>[2x]GPGSRYPVRRLPFSTVSKQDLAAFERIVPGGVVTDPEALQAPNVDWLRTLRGCSKVLLRPRTSEEVSHILRHCHERNLAVNPQGGNTGMVGGSVPVFDEIILSTARMNRVLSFHSVSGILVCQAGCVLEELSRYVEERDFIMPLDLGAKGSCHIGGNVATNAGGLRFLRYGSLHGTVLGLEVVLADGTVLDCLTSLRKDNTGYDLKQLFIGSEGTLGIITTVSILCPPKPRAVNVAFLGCPGFAEVLQTFSTCKGMLGEILSAFEFMDAVCMQLVGRHLHLASPVQESPFYVLIETSGSNAGHDAEKLGHFLEHALGSGLVTDGTMATDQRKVKMLWALRERITEALSRDGYVYKYDLSLPVERLYDIVTDLRARLGPHAKHVVGYGHLGDGNLHLNVTAEAFSPSLLAALEPHVYEWTAGQQGSVSAEHGVGFRKRDVLGYSKPPGALQLMQQLKALLDPKGILNPYKTLPSQAHHHHHH

Human D-2-HGDH is a member of the 2-hydroxy acid dehydrogenase subfamily of the VAO/PCMH flavoprotein family. Regardless of their promiscuous metabolic origins, D-2-HG and L-2-HG can be converted back to 2-OG by two mitochondrial enzymes in humans, namely D-2-HG and L-2-HG dehydrogenases (D-2-HGDH and L-2-HGDH). Like other members of the VAO/PCMH flavoprotein family, D-2-HGDH is comprised of two major domains named the FAD-binding domain and the substrate-binding domain supplemented with a small C-terminal domain. The active site resides at the interface of the FAD-binding domain and the substrate-binding domain, and consists of the FAD-binding site and the substrate-binding site.

In the apo structure, the substrate-binding site is occupied by several water molecules; in the D-2-HG-bound structure, there are a Zn2+ and a D-2-HG bound at the substrate-binding site. The structural comparison shows that the binding of Zn2+ and D-2-HG at the active site does not induce notable conformational changes in the overall structure and at the FAD-binding site, and hence does not affect the conformation of FAD and its interactions with the protein. The structural comparison shows that the binding of Zn2+ and D-2-HG does not induce notable conformational changes at the substrate-binding site as well except for Glu475 which adopts a different side-chain conformation to interact with the Zn2+. The Zn2+ is coordinated by six ligands, including the side chains of His434, His441, and Glu475, the O4 atom of FAD, and the C1-carboxyl and C2-hydroxyl of D-2-HG. The lactate moiety of D-2-HG is positioned in parallel to the isoalloxazine ring of FAD and the acetate moiety is extended into the deep end of the substrate-binding pocket; both moieties are recognized by several conserved residues. Specifically, the C1-carboxyl of D-2-HG forms several hydrophilic interactions with the side chains of Arg386, Thr390, His434, and His441, two hydrogen bonds with the O4 atom of FAD and a water molecule (Wat1), and a coordination bond with the Zn2+. The C2-hydroxyl of D-2-HG forms hydrogen bonds with the side chains of His441, Glu475, and His476, and a coordination bond with the Zn2+. The C5-carboxyl of D-2-HG forms a salt bridge with the side chain of Lys401 and four hydrogen bonds with the side chains of Thr390, Tyr432, and Asn443, and a water molecule (Wat2). In particular, the O4 atom of the isoalloxazine ring is involved in the coordination of Zn2+ and forms two hydrogen bonds with the C1-carboxyl of D-2-HG and a water molecule (Wat1), and the O2 atom forms three hydrogen bonds with the main-chain amine of Gly209, the side chain of Glu475, and a water molecule (Wat3).> GCCS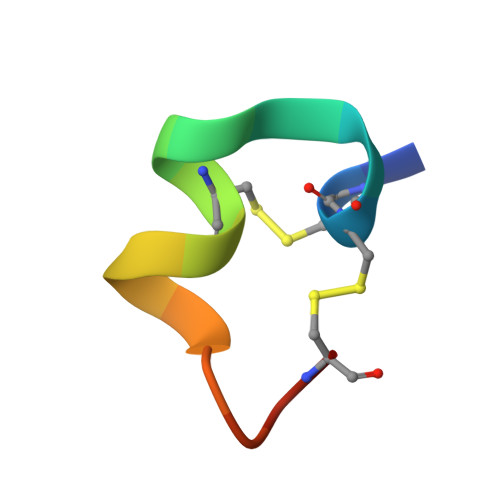RPPCILNNPDLCX>MTTLTARPEAITFDPQQSALIVVNMQNAYATPGGYLDLAGFDVSTTRPVIANIQTAVTAARAAGMLIIWFQNGWDEQYVEAGGPGSPNFHKSNALKTMRKQPQLQGKLLAKGSWDYQLVDELVPQPGDIVLPKPRYSGFFNT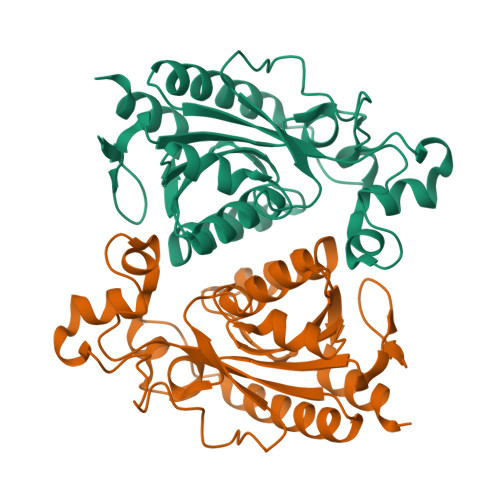PLDSILRSRGIRHLVFTGIATNVCVESTLRDGFFLEYFGVVLEDATHQAGPKFAQKAALFNIETFFGWVSDVETFCDALSPTSFAHIA[8x]>GSKKLINDVQDVLDEQLAGLAKAHPSLTLHQDPVYVTRADAPVAGKVALLSGGGSGNEPMHCGYIGQGMLSGACPGEIFTSPTPDKIFECAMQVDGGEGVLLIIKNYTGDILNFETATELLHDSGVKVTTVVIDDDVAVKDSLYTAGRRGVANTVLIEKLVGAAAERGDSLDACAELGRKLNNQGHSIGIALGACTVPAAGKPSFTLADNEMEFGVGIHGEPGIDRRPFSSLDQTVDEMFDTLLVNGSYHRTLRFWDYQQGSWQEEQQTKQPLQSGDRVIALVNNLGATPLSELYGVYNRLTTR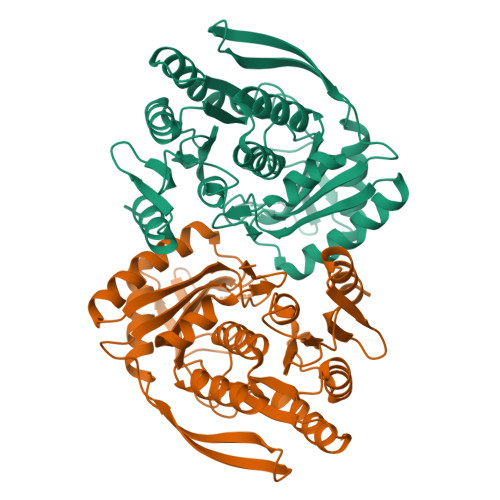CQQAGLTIERNLIGAYCTSLDMTGFSITLLKVDDETLALWDAPVHTPALNWGK[4x]(2S,3S,4R,5R)-5-(6-AMINOPURIN-9-YL)-N-[[(2S,3S,4R,5R)-5-(2,4-DIOXOPYRIMIDIN-1-YL)-4-HYDROXY-2-(HYDROXYMETHYL)OXOLAN-3-YL]METHYLSULFONYL]-3,4-DIHYDROXY-OXOLANE-2-CARBOXAMIDE | C20 H28 N8 O11 S 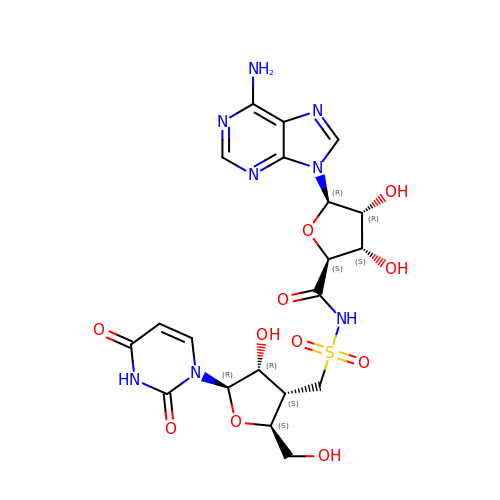| KEQMCGJHYDWPEW-ZSIUBJGCSA-N>MARNIVVEEIVRTPVEMQQVELVERKGIGHPDSIADGIAEAVSRALCREYIRRYGVILHHNTDQVE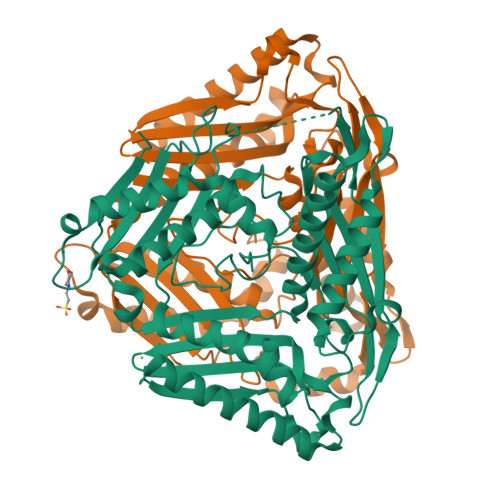VVGGRAYPRFGGGEVVKPIYILLSGRAVELVDQELFPVHEVAIKAAKNYLKNAIRHLDVENHVIIDSRIGQGSVDLVSVFNKARENPIPLANDTSFGVGYAPLSETERLVLETEKLLNSEKFKKEYPAVGEDIKVMGLRRGNEIDLTIAAAIVDSEVATPKEYLEVKDKIKEAVEELAKEITSRKVNIYVNTADDPERGIYYITVTGTSAEAGDDGSVGRGNRVNGLITPNRHMSMEAAAGKNPVSHVGKIYNILAMLIAEDIAKTLPVEEVYVRILSQIGKPIDQPLVASIQVIPKPGHSVKEFEKDAYSIADEWLANITKVQKMILEDKISVF[4x]>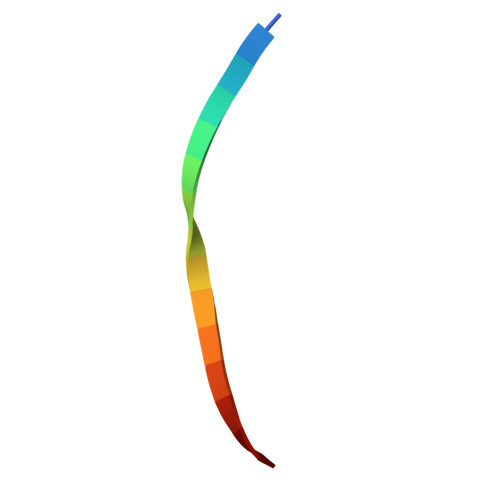 ADSIEIYIPEAQTRL3-(8-amino-3,4-dihydroisoquinolin-2(1H)-yl)-N-methylpropanamide | C13 H19 N3 O | 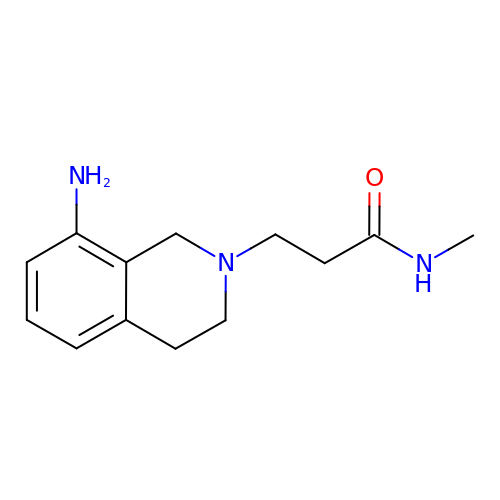RZXHZFVCPWDPAP-UHFFFAOYSA-N>DVTNAEKLVYKY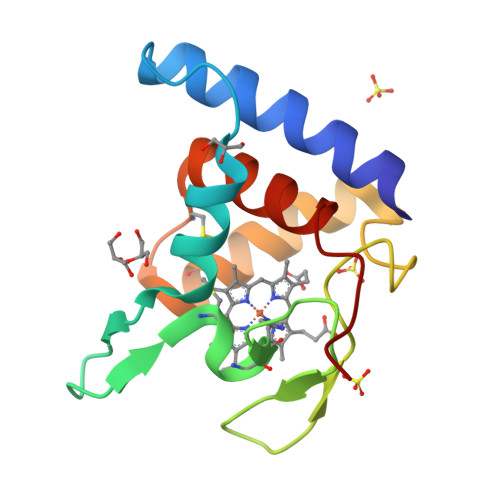TNIAHSANPMYEAPSITDGKIFFNRKFKTPSGKEAACASCHTNNPANVGKNIVTGKEIPPLAPRVNTKRFTDIDKVEDEFTKHCNDILGADCSPSEKANFIAYLLTETKPTK[2x]>[4x]MNLKDKILGVAKELFIKNGYNATTTGEIVKLSESSKGNLYYHFKTKENLFLE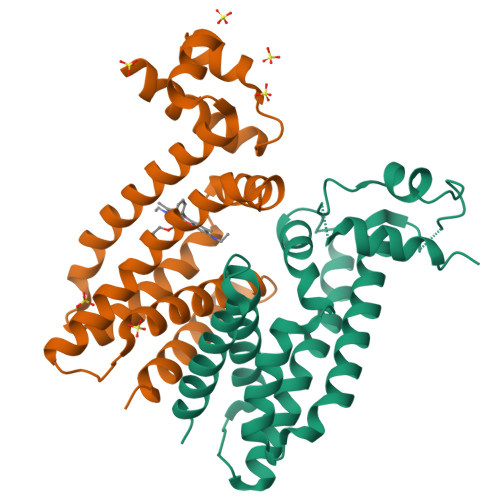ILNIEESKWQEQWKSEQIKAKTNREKFYLYNELSLTTEYYYPLQNAIIEFYTEYYKTNSINEKMNKLQNKYIDAYHVIFKEGNLNGEWSINDVNAVSKIAANAVNGIVTFTHEQNINERIKLMNKFSQIFLNGLSKHHHHHH>[7x]MASDISKCFATLGATLQDSIGKQVLVKLRDSHEIRGILR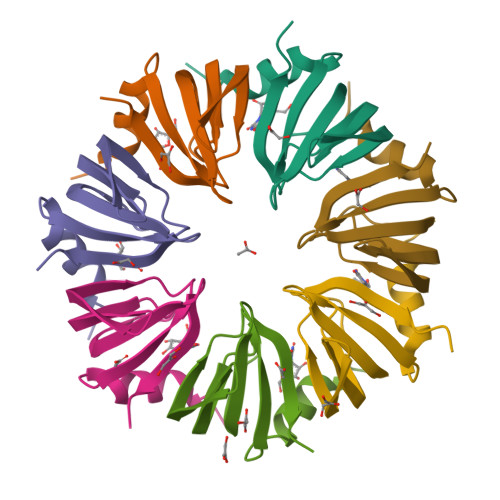SFDQHVNLLLEDAEEIIDGNVYKRGTMVVRGENVLFISPVPG> XTDAVLELPAATFDLPLSLSGGTQTTLRAHAGHWLVIYFYPKDSTPGCTTEGLDFNALLPEFDKAGAKILGVSRDSVKSHDNFSAKQGFAFPLVSDGDEALCRAFDVIKEKNMYGKQVLGIERSTFLLSPEGQVVQAW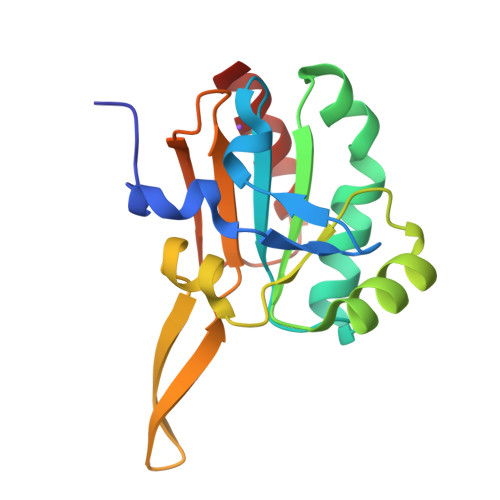RKVKVAGHADAVLAALKAHAKQ> MSEESQAFQRQLTALIGYDVTDVSNVHDDELEFTRRGLVTPRMAEVASRDPKLYAMHPWVTSKPLPEYLWKKIANNCIFIVIHRSTTSQTIKVSPDDTPGAILQSFFTKMAKKKSLMDIPESQSEQDFVLRVCGRDEYLVGETPIKNFQWVRQCLKNGEEIHVVLDTPPDPALDEVRKEEWPLVDDCTGVTGYHEQLTIHGKDHESVFTVSLWDCDRKFRVKIRGIDIPVLPRNTDLTVFVEANIQHGQQVLCQRRTSPKPFTEEVLWNVWLEFSIKIKDLPKGALLNLQIYCGKAPALSSKASAESPSSESKGKVQLLYYVNLLLIDHRFLLRRGEYVLHMWQISGKGEDQGSFNADKLTSATNPDKENSMSISILLDNYCHPIALPKHQPTPDPEGDRVRAEMPNQLRKQLEAIIATDPLNPLTAEDKELLWHFRYESLKHPKAYPKLFSSVKWGQQEIVAKTYQLLARREVWDQSALDVGLTMQLLDCNFSDENVRAIAVQKLESLEDDDVLHYLLQLVQAVKFEPYHDSALARFLLKRGLRNKRIGHFLFWFLRSEIAQSRHYQQRFAVILEAYLRGCGTAMLHDFTQQVQVIEMLQKVTLDIKSLSAEKYDVSSQVISQLKQKLENLQNLNLPESFRVPYDPGLKAGALAIEKCKVMASKKKPLWLEFKCADPTALSNETIGIIFKHGDDLRQDMLILQILRIMESIWETESLDLCLLPYGCISTGDKIGMIEIVKDATTIAKIQQSTVGNTGAFKDEVLNHWLKEKSPTEEKFQAAVERFVYSCAGYCVATFVLGIGDRHNDNIMITETGNLFHIDFGHILGNYKSFLGINKER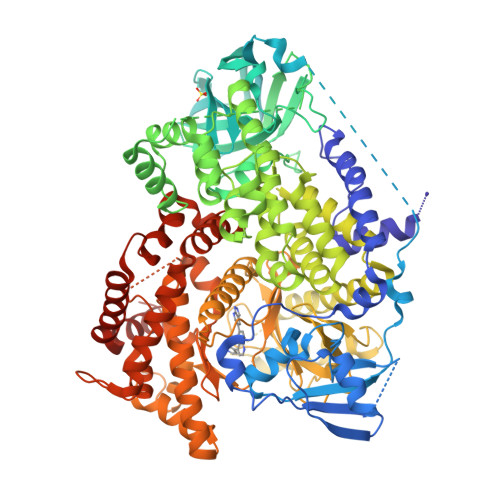VPFVLTPDFLFVMGTSGKKTSPHFQKFQDVCVKAYLALRHHTNLLIILFSMMLMTGMPQLTSKEDIEYIRDALTVGKNEEDAKKYFLDQIEVCRDKGWTVQFNWFLHLVLGIKQGEKHSAHHHHHH> CPEQDKYRTITGMCNNRRSPTLGASNRAFVRWLPAEYEDGFSLPYGWTPGVKRNGFPVALARAVSNEIVRFPTDQLTPDQERSLMFMQWGQLLDHDLDFTPEPAARASFVTGVNCETSCVQQPPCFPLKIPPNDPRIKNQADCIPFFRSCPACPGSNITIRNQINALTSFVDASMVYGSEEPLARNLRNMSNQLGLLAVNQRFQDNGRALLPFDNLHDDPCLLTNRSARIPCFLAGDTRSSEMPELTSMHTLLLREHNRLATELKSLNPRWDGERLYQEARKIVGAMVQIITYRDYLPLVLGPTAMRKYLPTYRSYNDSVDPRIANVFTNAFRYGHTL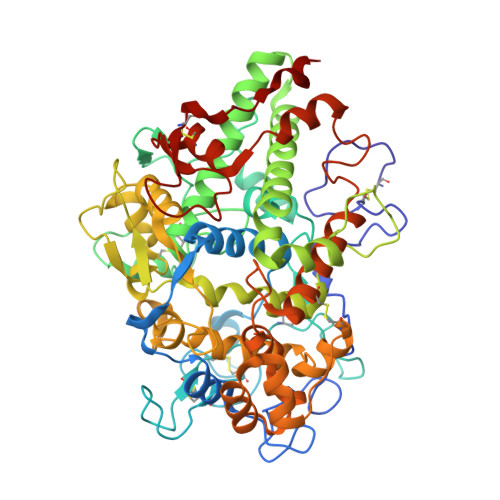IQPFMFRLDNRYQPMEPNPRVPLSRVFFASWRVVLEGGIDPILRGLMATPAKLNRQNQIAVDEIRERLFEQVMRIGLDLPALNMQRSRDHGLPGYNAWRRFCGLPQPETVGQLGTVLRNLKLARKLMEQYGTPNNIDIWMGGVSEPLKRKGRVGPLLACIIGTQFRKLRDGDRFWWENEGVFSMQQRQALAQISLPRIICDNTGITTVSKNNIFMSNSYPRDFVNCSTLPALNLASWRE AppA, the Escherichia coli periplasmic phytase of clade 2 of the histidine phosphatase (HP2) family, has been well-characterized and successfully engineered for use as an animal feed supplement. The E. Coli periplasmic phytase, AppA, is a 1D-6-phytase (EC 3.1.3.2) and initial hydrolysis preferentially liberates the phosphate at the 1D-6-position on the inositol ring. HP2Ps catalyse the hydrolysis of phytate via an obligatory phosphohistidine intermediate. The catalytic proton donor is found in a second, short, conserved motif with sequence HD positioned such that the aspartic acid residue functions as the consensus proton donor in the catalytic mechanism.

KM also decreased for the AppA-HDE mutant while its turnover number is reduced to ~17% of the wild-type enzyme. Only AppA-HDE showed an increase in stereospecificity, decreasing the production of InsP5 [1/3-OH] to only 6% of total InsP5. In addition, while AppA-HDE increased specificity towards InsP6 relative to the wild-type enzyme, it showed reduced accumulation of 1D-myo-Ins(2,3,4,5)P4, accumulating instead a novel InsP2 intermediate. On the contrary, the variant AppA-HDE becomes more stereospecific than the wild type while reducing the accumulation of the 1D-myo-Ins(2,3,4,5)P4 intermediate. Despite its lower catalytic efficiency, this variant is a good candidate for further investigation into its potential for use in animal feeds. At residue position 305, the T305E substitution found in the AppA-HDE and -HAE variants results in sidechain χ1 angles of 46° and 65°, respectively, for the glutamate residue. Thus, in the AppA-HAE and -HDE variants the E305 sidechain points away from the substrate and towards the active site cavity. AppA-HDE has slightly enlarged pockets A and B due to the loss of the side-chain methyl group of T305, whereas the double mutant AppA-HAE has larger pockets A and B with an overall change in polarity. For both variants, pocket F decreases in size and its polarity increases by virtue of introduction of the larger sidechain of and carboxyl group of glutamate. In particular, active site comparisons suggest that an enlargement of specificity pocket B allows accommodation of multiple InsS6 binding poses (e.g., for AppA-HET), while the decrease in size of pocket F by the substitution T305E (e.g., AppA-HDE) leads to an enhancement of stereospecificity.

> GPQSEPELKLESVVIVSRHGVRAPTKATQLMQDVTPDAWPTWPVKLGWLTPRGGELIAYLGHYQRQRLVADGLLAKKGCPQSGQVAIIADVDERTRKTGEAFAAGLAPDCAITVHTQADTSSPDPLFNPLKTGVCQLDNANVTDAILSRAGGSIADFTGHRQTAFRELERVLNFPQSNLCLKREKQDESCSLTQALPSELKVSADNVSLTGAVSLASMLTEIFLLQQAQGMPEPGWGRITDSHQWNTLLSLHNAQFYLLQRTPEVARSRATPLLDLIKTALTPHPPQKQAYGVTLPTSVLFIAGHDENLANLGGALELNWTLPGQPDNTPPGGELVFERWRRLSDNSQWIQVSLVFQTLQQMRDKTPLSLNTPPGEVKLTLAGCEERNAQGMCSLAGFTQIVNEARIPACSL>GSHMGTKNIGKGLTFEDILLVPNYSEVLPREVSLETKLTKNVSLKIPLISSAMDTVTEHLMAVGMARLGGIGIIHKNMDMESQVNEVLKVKNSGGLRVGAAIGVNEIERAKLLVEAGVDVIVLDSAHGHSLNIIRTLKEIKSKMNIDVIVGNVVTEEATKELIENGADGIKVGIGPGSICTTRIVAGVGVPQITAIEKCSSVASKFGIPIIADGGIRYSGDIGKALAVGASSVMIGSILAGTEE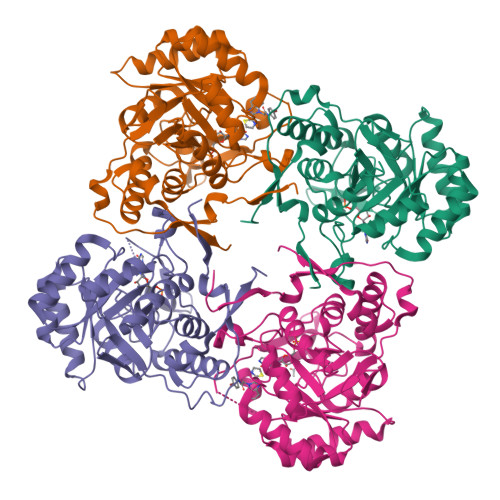SPGEKELIGDTVYKYYRGMGSVGAMKSGSGDRYFQEKRPENKMVPEGIEGRVKYKGEMEGVVYQLVGGLRSCMGYLGSASIEELWKKSSYVEITTSGLRESHVHDVEIVKEVMNYSK[8x]N-{[(2R,3R,4R,5R)-3,4-DIHYDROXY-5-(HYDROXYMETHYL)PYRROLIDIN-2-YL]METHYL}-4-(DIMETHYLAMINO)BENZAMIDE | C15 H23 N3 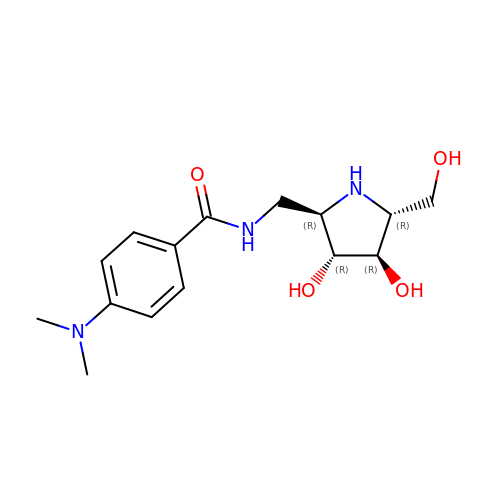O4 | OULLPOCYJLHTGG-AAVRWANBSA-N>[4x]MAISKTNGQSKPKRKTEVPGQALGYSLQFTLLTHLLLQAPEGSLCSLEVLDDVAQENNSGDIKFIQSASALTANPAADRAKSLWKTLSNWIDLATSPDFEVEKAIFELYVSRPVEGSIVKKFNEAKTPEDAQEAITHARTELWGDS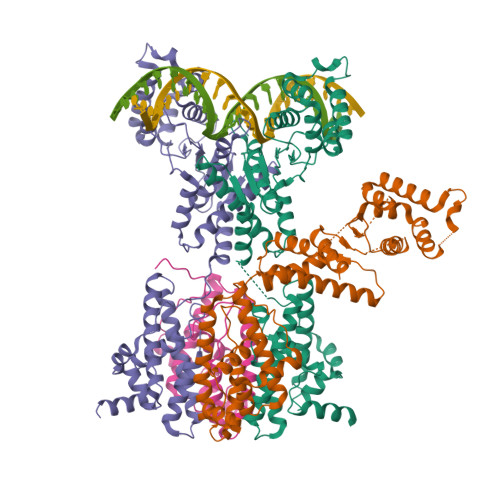PHFTLKDGISKEISKYVEKVFTADQNLLQRLICNFQLTLGSGSPQADLEACVRSHPVSPSKVSDITNYLCGKVKRHIDMLLEAEKPAVIARDDFYTWYKAYVQKIDRQMVLSSRAQAPVKEKAQEYLPDKFVQQLEIIGLPYEEILGAISDYLMASFDRTDWAARGEVDETSFDDLDTALQRTWKNKQRICGLTHSEKSEQDQGKLLYFECMQFNIPLQAMSPPSHFIPGCYHILADSLAVGWHPNYTTQLKNKKVA>[3x]GNSDCYFGNGSAYRGTHSLTESGA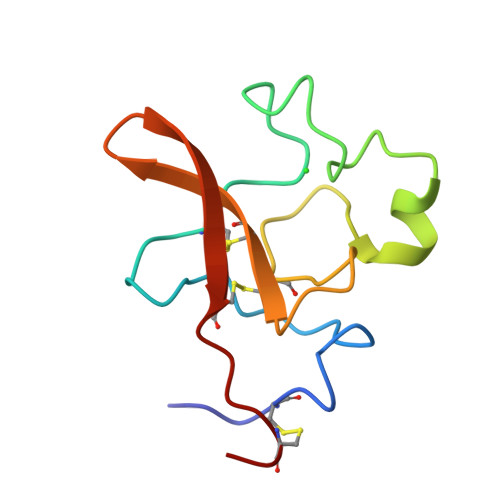SCLPWNSMILIGKVYTAQNPSAQALGLGKHNYCRNPDGDAKPWCHVLKNRRLTWEYCDVPSCST>[6x]MTDIVYDVEGFRAFLPKETLRWIRHRELERKVGVVEKFSDRVGPIPVEIRRRRSQYGEFYHAGKGTTRIQARVSAAMECVERAAAEPREEIIERGPEGDKWTPAWYRTEPREWVEGVDLTTREPVYVPANEVF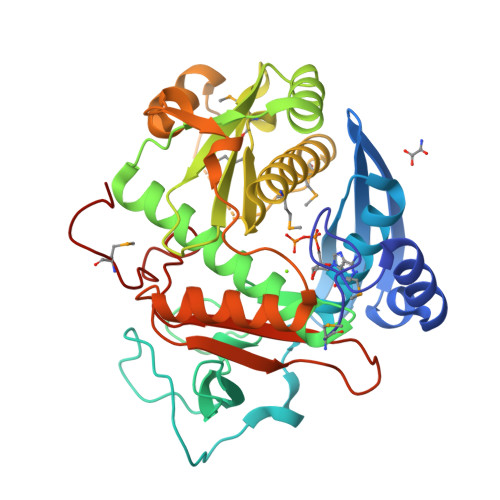HPWLGDALPSHTNGLSAGRLREEAVIQGLLEVVERDSWSIVEYFRIHPPELEVHGELEELRRSLEREVGRVELRLLPSRVEGVYVVGAVTEAERVEEMVMGFGASPDPEMAVLRALLEVAQGLSMARRGIESPVRKGLGEFSAPGKLTPERLKRLNRHWFEPEGTVEIDDLDRVITTGSLEKLTEELVERVAEAGLGKVIEVDLTLENLDVPVVRVRVTGASEYVIDEARVGNMPEKPPGVPMG> GGGIDYIKLLGEIATENQFEVTYVDIEEKTFSGQFQC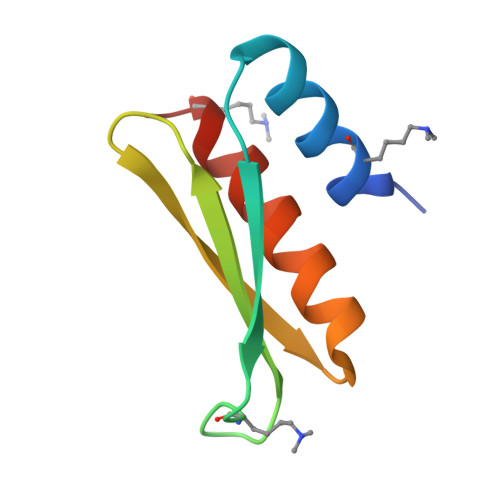LVQLSTLPVGVCHGSGPTAADAQRHAAQNALEYLKIMT1-[3-tert-butyl-1-(4-methylphenyl)-1H-pyrazol-5-yl]-3-[2-(morpholin-4-yl)ethyl]urea 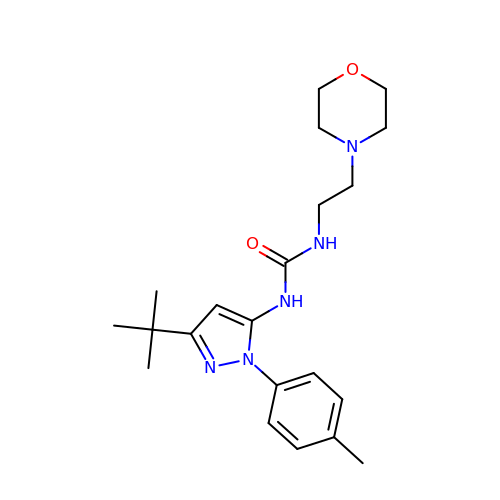| C21 H31 N5 O2 | WTTXDKWUUKCBRY-UHFFFAOYSA-N> MDRRALRIGVNGLPPSLEPINGISNTGPRIINQIFDALIRRDYFADGAKGNNIKLVPALAESFERIDDKSIRFKLRQGVKFHNGAEMTAEDVAFTFSSERLWGDEAIKTVPNGRNFSPNWDEPVVEDKYTVVLRTKTPSYLIEKYLGSWLGPIVPKEYYKSLGAVAFGNKPIGTGPYKFRELVANDHVTLEANDGYWGDKPTASTITYQVVAEPATRVAGLISGEYDIITTLTPDDMALVDGYSDLETRGTLIENLHMFTFNMNQPIFQNKTLRRALALAVNRPLIVEALWKNKASIPNGFNFPHYGATYDPKRKPMEFNLKEAKR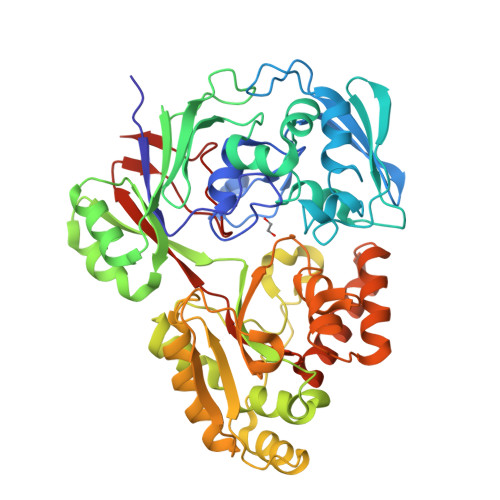LVKESGYDGTPITYHTMGNYYANAVPALMMMIEMWKAAGITVVPKIFAPGTTPKDSDILIRNWSNGQWLTDGLTTMVSEFGPGRGVQKRWGWKAPAEFNNLCDQVAQLKDGEERSAAFNRLRDIFEDEAPAVLMYQPYDVYAARKDVQWSPVSFETMEFRGNLNFKHHHHHH>[2x]KIRIGINGFGRIGRLVARVVLQRDDVELVAVNDPFITTEYMTYMFKYDSVHGQWKHNELKIKDEKTLLFGEKPVTVFGIRNPEDIPWAEAGADYVVESTGVFTDKDKAAAHLKGGAKKVVISAPSKDAPMFVVGVNEHEYKSDLDIVSNASCTTNCLAPLAKVINDRFGIVEGLMTTVHSITATQKTVDGPSMKDWRGGRAASFNIIPSSTGAA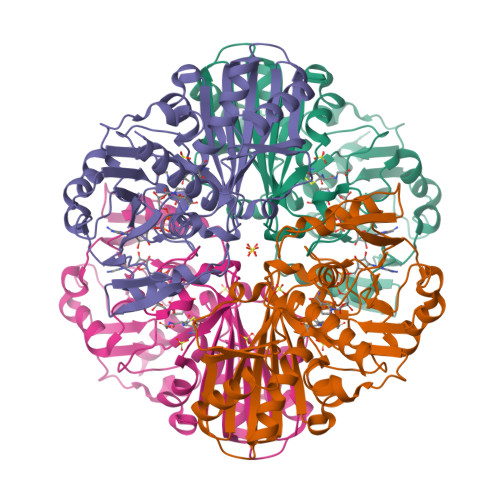KAVGKVLPALNGKLTGMSFRVPTVDVSVVDLTVRLEKAATYDEIKKAIKEESEGKLKGILGYTEDDVVSTDFVGDNRSSIFDAKAGIALSDKFVKLVSWYDNEWGYSSRVVDLIVHMSKA> RVADTVGTGPTNSEAIPALTAAETGHTSQVVPGDTMQTRHVKNYHSRSESTIENFLCRSACVYFTEYKNSGAKRYAEWVLTPRQAAQLRRKLEFFTYVRFDLELTFVITSTQQPSTTQNQDAQILTHQIMYVPPGGPVPDKVDSYVWQTSTNPSVFWTEGNAPPRMSIPFLSIGNAYSNFYDGWSEFSRNGVYGINTLNNMGTLYARHVNAGSTGPIKSTIRIYFKPKHVKAWIPRPPRLCQYEKAKNVNFQPSGVTTTRQSITTMTNT;> SDRARSITLGNSTITTQECANVVVGYGVWPDYLKDSEATAEDQPTQPDVATCRFYTLDSVQWQKTSPGWWWKLPDALSNLGLFGQNMQYHYLGRTGYTVHVQCNASKFHQGCLLVVCVPEAEMGCATLDNTPSSAELLGGDTAKEFADKPVASGSNKLVQRVVYNAGMGVGVGNLTIFPHQWINLRTNNSATIVMPYTNSVPMDNMFRHNNVTLMVIPFVPLDYCPGSTTYVPITVTIAPMCAEYNGLRLAG;> GLPTMNTPGSCQFLTSDDFQSPSAMPQYDVTPEMRIPGEVKNLMEIAEVDSVVPVQNVGEKVNSMEAYQIPVRSNEGSGTQVFGFPLQPGYSSVFSRTLLGEILNYYTHWSGSIKLTFMFCGSAMATGKFLLAYSPPGAGAPTKRVDAMLGTHVIWDVGLQSSCVLCIPWISQTHYRFVASDEYTAGGFITCWYQTNIVVPADAQSSCYIMCFVSACNDFSVRLLKDTPFISQQNFF;> GAQVSTQKTGAHETRLNASGNSIIHYTNINYYKDAASNSANRQDFTQDPGKFTEPVKDIMIKSLPALN

The protomers assemble to form the ∼30 nm wide icosahedral shell with a pseudo T = 3 arrangement that encapsidates the linear single-stranded RNA genome. The arrangement occurs because of the similar structures of VP1, VP2, and VP3, which all adopt an eight-stranded, antiparallel β-barrel fold despite having low sequence homology. Recently, we discovered a second druggable pocket at a conserved VP1–VP3 interprotomer interface in the viral capsid. Here, in an effort to better understand the druggable features of the interprotomer pocket, we have analyzed high-resolution structures of two medically important enteroviruses, coxsackieviruses B3 and B4, complexed with interprotomer-targeting compounds CP17 and CP48, respectively.

CP17 is a benzenesulfanomide derivative that potently inhibits the CVB3 Nancy strain in cells (EC50 0.7 ± 0.1 µM) via a direct interaction with the capsid that increases virion thermostability by 1.5 and 2.1 log10 TCID50/mL at 46 and 49 °C, respectively. A 4.0 Å cryo-EM structure of CP17 in complex with CVB3 Nancy (EMD-0103) revealed that the site of binding is located at a conserved VP1–VP3 interprotomer interface, but the low resolution of the map prevented identification of the detailed interactions within the pocket. We reprocessed the raw data (EMPIAR-10199) using RELION 3.0 and the resolution improved to 2.8 Å. The cryo-EM map shows pronounced backbone features for the four structural proteins of CVB3, and well-defined density for CP17 on the surface of the capsid. The interprotomer site is located between adjacent asymmetric units “protomers” in a narrow opening formed at the intersection of neighboring VP1 β-barrels and the C terminus of a proximally situated VP3 molecule. Three residues that play a key role in binding CP17 are conserved across enteroviruses. In CVB3 Nancy they are Arg219 (VP1), Arg234 (VP1), and Gln233 (VP3). The Arg residues, which come from neighboring VP1 polypeptide chains, are situated in the deepest part of the pocket, and in the high-resolution structure, we observed that their guanidinium groups form salt bridges with the carboxylic end of CP17. The Gln residue from the C terminus of VP3 is positioned at the entrance of the drug site, where the oxygen in the side chain engages in a hydrogen bond interaction with the NH located in the elbow region of the inhibitor. In addition, there are other contributions inside the pocket such as a cysteine residue in VP1 (C73) and hydrophobic residues (VP1 F76 and VP3 F236) that interact with the benzene rings of the compound, contributing to the overall binding energy and specificity of CP17.> IVGGKVCPKGECPWQVLLLVNGAQLCGGTLINTIWVVSAAHCFDKIKNWRNLIAVLGEHDLSEHDGDEQSRRVAQVIIPSTYVPGTTNHDIALLRLHQPVVLTDHVVPLCLPERTFSERTLAFVRFSLVSGWGQLLDRGATALELMVLNVPRLMTQDCLQQSRKVGDSPNITEYMFCAGYSDGSKDSCKGDSGGPHATHYRGTWYLTGIVSWGQGCATVGHFGVYTRVSQYIEWLQKLMRSEPRPGVLLRAPFP;> ANAFLEELRPGSLERECKEEQCSFEEAREIFKDAERTKLFWISYSDGDQCASSPCQNGGSCKDQLQSYICFCLPAFEGRNCETHKDDQLICVNENGGCEQYCSDHTGTKRSCRCHEGYSLLADGVSCTPTVEYPCGKIPILEKRNASKPQGR;> NTVAAYNLTWKSTNFKTILEWEPKPVNQVYTVQISTKSGDWKSKCFYTTDTECDLTDEIVKDVKQTYLARVFSYPAGNVE;> GEPLYENSPEFTPYLETNLGQPTIQSFEQVGTKVNVTVEDERTLVRRNNTFLSLRDVFGKDLIYTLYYWKSSSSGKKTAKTNTNEFLIDVDK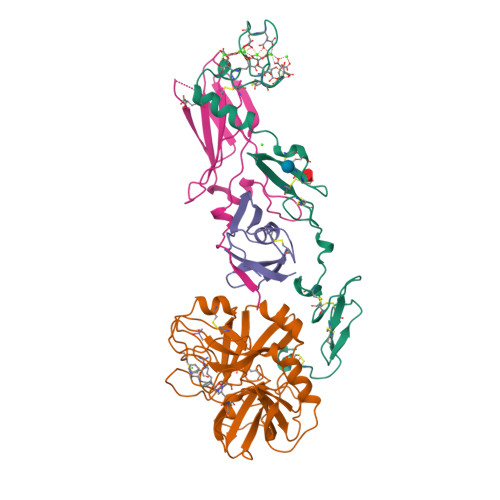GENYCFSVQAVIPSRTVNRKSTDSPVECM>[2x]MLSLNNLQNIIYNPVIPFVGTIPDQLDPGTLIVIRGHVPSDADRFQVDLQNGSSVKPRADVAFHFNPRFKRAGCIVCNTLINEKWGREEITYDTPFKREKSFEIVIMVLKDKFQVAV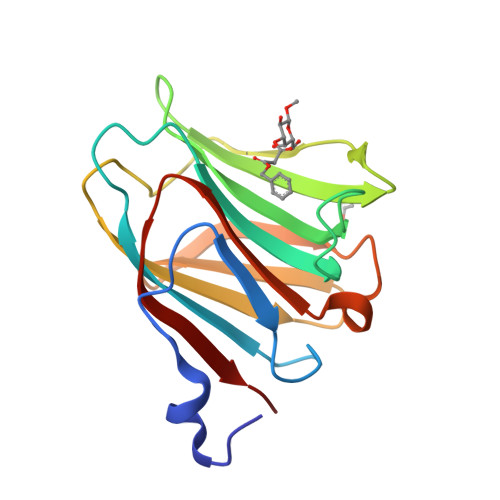NGKHTLLYGHRIGPEKIDTLGIYGKVNIHSIGFSFS>LDNGLARTPTMGWLHWERFMCNLDCQEEPDSCISEKLFMEMAELMVSEGWKDAGYEYLCIDDCWMAPQRDSEGRLQADPQRFPHGIRQLANYVHSKGLKLGIYADVGNKTCAGFPGSFGYYDIDAQTFADWGVDLLKFDGCYCDSLENLADGYKHMSLALNRTGRSIVYSCEWPLYMWPFQKPNYTEIRQYCNHWRNFADIDDSWKSIKSILDWTSFNQERIVDVAGPGGWNDPDMLVIGNFGLSWNQQVTQMALWAIMAAPLFMSNDLRHISPQAKALLQDKDVIAINQDPLGKQGYQLRQGDNFEVWERPLSGLAWAVAMINRQEIGGPRSYTIAVASLGKGVACNPACFITQLLPVKRKLGFYEWTSRLRSHINPTGTVLLQLENTMQMSLKDLL[2x]

α-Galactosidase A (α-Gal A, EC 3.2.1.22) is a lysosomal glycosidase that hydrolyzes the terminal α-linked galactoside present on macromolecules such as globotriaosylceramide (Gb3).1,2 Mutations in the α-galactosidase A gene (GLA) are found in patients with Fabry disease (FD), one of the most common lysosomal storage diseases (LSDs), which is characterized by the progressive accumulation of Gb3 in cells. To unravel the binding mechanism of iminosugars with α-Gal A, N-methylated derivatives 20–24 were synthesized, and we determined the crystal structures of α-Gal A in complex with compounds 4 and 5 at pH 7.2 and 4.5, respectively, and 8, 20, 21, 23, and 24 at pH 7.2 at 1.97 to 2.61 Å resolution.2,32 The structures revealed that these pyrrolidines bind to the catalytic site nearly in the center of the TIM-barrel domain of the enzyme. The bindings are primarily stabilized not only by hydrogen bonds (H-bonds) between the hydroxyl groups of the compounds and the residues D92, D93, L168, D170, E203, R227, and D231 of α-Gal A but also by a salt bridge between the endocyclic amino group (endo-N) of the monobasic compounds (pKa ∼ 7.0) and D170 of the enzyme at pH 7.2.

Previously, the dibasic iminosugar and potent α-Gal A inhibitor 5 having the (2R,3R,4S,5R) configuration pattern demonstrated good chaperoning activity in cells transiently transfected with various mutant α-Gal A.23 Notably, iminosugar 5 exhibited superior pH-dependence in its inhibitory activity compared to its monobasic parent molecule, 4, suggesting that it binds to α-Gal A at pH 7.0 more effectively than 4, leading to better enzyme-stabilizing or chaperoning activity. Surprisingly, in the compound 5-bound structure of α-Gal A, the positively charged exocyclic amino group (exo-N, pKa = 9.1) of 5 forms bifurcated salt bridges (BSBs) with residues E203 and D231 of the enzyme at pH 7.2, where the carboxylic side chains are essentially deprotonated and negatively charged. By contrast, the corresponding C-2 hydroxyl group of 4 forms H-bonds alone to E203 and D231 at pH 7.2. This finding most likely reflects the stronger binding affinity and better protecting effects of 5 toward α-Gal A at pH 7.2 compared to those of 4. In contrast, the titration curves revealed that the endo-N moiety in compound 5 exhibits reduced basicity (pKa = 5.5) compared to that of 4 (pKa = 7.0) due to electrostatic repulsion between the vicinal ammonium cations,34 which implies the formation of an H-bond between endo-N of 5 and D170 at pH 7.0 but a salt bridge at pH 4.5. Given these structural findings, it is conceivable that the pH-dependent protonation states on the amino groups of iminosugars and ionizable residues in the catalytic site of α-Gal A regulate the binding status of the compounds, i.e., the stronger binding of 5 to α-Gal A at pH 7.2 is due to the formation of the BSBs, which are missing at pH 4.5 when the binding is weaker and only H-bonds are formed.The CP is capped by a 19S regulatory particle (RP) that houses three ubiquitin-binding substrate receptors, Rpn1, Rpn10 and Rpn132. A pleckstrin-like receptor for ubiquitin (Pru) domain in hRpn13 binds ubiquitin and proteasome subunit hRpn2. hRpn13 Pru binds proteasomes at the extreme C-terminus of hRpn2, which is otherwise intrinsically disordered. Here, we report that hRpn13 Pru also acts as a generalized peptide-binding domain.

Crystals were obtained for hRpn13 in the absence of ligands that diffracted to 1.85 Å resolution with one hRpn13 molecule per asymmetric unit. We tested and found that the electron density fit well to the extreme N-terminal (ENT) amino acids, which we define as including the residual G-P-G-S sequence (aG-bP-cG-dS) of the purification tag and M1 – T3 of the native hRpn13 sequence. ENT forms a U-shaped structure with the non-native sequence along one side and the native sequence along the other (yellow and orange, respectively). ENT forms hydrophobic contacts with hRpn13 Pru M1 at the valley of the U structure surrounded by P40, S90 and W108. These amino acids are similarly involved in proteasome binding by interacting with hRpn2 P945 and E946. At the U hinge, a bound water bridges native and non-native amino acids by forming hydrogen bonds with the dS and M1 backbone amide groups and sidechain oxygen of T2. Analysis of ENT in the context of the neighboring asymmetric unit supports this hypothesis, as ENT M1 interacts with the W108-containing surface ( ) of one hRpn13 molecule, named Pru-A, and the F76-containing surface of the neighboring molecule, named Pru-B. The sidechain oxygen and nitrogen atoms of Pru-B D78 and K99 form hydrogen bonds with the main chain cG amide nitrogen and aG carbonyl oxygen, respectively (insert). Between ENT and Pru are 16 residues that span S4 – N20, which are not present in the electron density map.

> MTTSGALFPSLVPGSRGASNKYLVEFRAGKMSLKGTTVTPDKRKGLVYIQQTDDSLIHFCWKDRTSGNVEDDLIIFPDDCEFKRVPQCPSGRVYVLKFKAGSKRLFFWMQEPKTDQDEEHCRKVNEYLNNPPMPGALGASGSSGHELSAL;> GPGSMTT2-propyl[1,3]thiazolo[4,5-c]quinolin-4-amine | C13 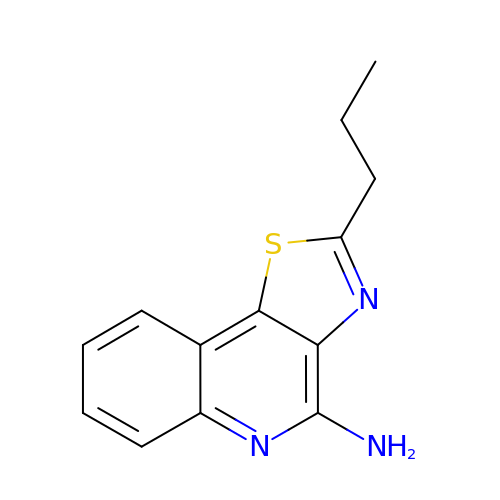H13 N3 S | NFYMGJSUKCDVJR-UHFFFAOYSA-N>[2x]MK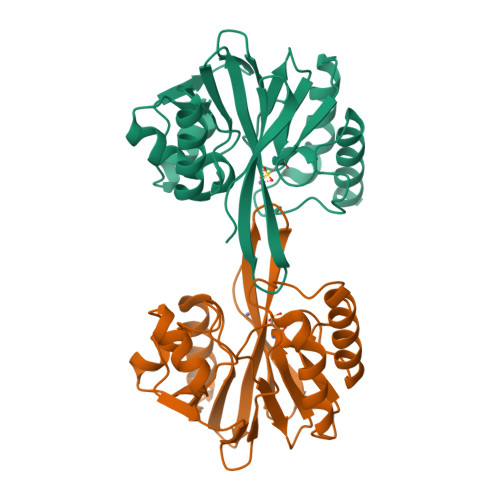NVLVFLILLVALPALAQGHKPLEVIKIEDGVYLHTSFKNIEGYGLVDSNGLVVLDNNQAYIIDTPWSEEDTKLLLSWATDRGYQVMASISTHSHEDRTAGIKLLNSKSIPTYTSELTKKLLAREGKPVPTHYFKDDEFTLGNGLIELYYPGAGHTEDNIVAWLPKSKILFGGCLVRSHEAEGLGYVGDASISSWADSIKNIVSKKYPIQMVVPGHGKVGSSDILDHTIDLAESASNKLMQPTAEASAD> AEIGGDHGYNATNIA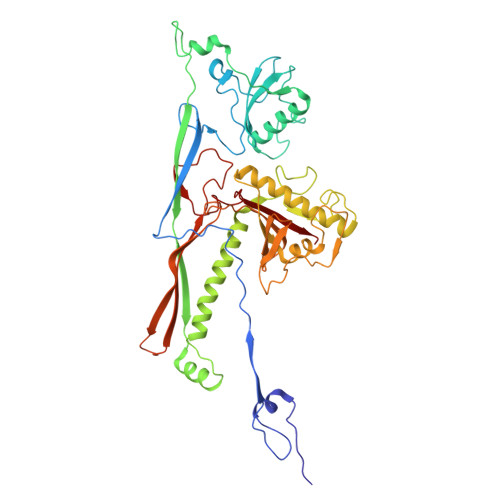AGQTSGAVTQIGPAVMGMVRRAIPNLIAFDICGVQPMNSPTGQVFALRAVYGKDPVAAGAKEAFHPMYGPDAMFSGQGAAKKFPALAASTQTTVGDIYTHFFQETGTVYLQASVQVTIDAGDEDEDEDEDATDAAKLDAEIKKQMEAGALVEIAEGMATSIAELQEGFNGSTDNPWNEMGFRIDKQVIEAKSRQLKAAYSIELAQDLRAVHGMDADAELSGILATEIMLEINREVVDWINYSAQVGKSGMTLTPGSKAGVFDFQDPIDIRGARWAGESFKALLFQIDKEAVEIARQTGRGEGNFIIASRNVVNVLASVDTGISYAAQGLATGFSTDTTKSVFAGVLGGKYRVYIDQYAKQDYFTVGYKGPNEMDAGIYYAPYVALTPLRGSDPKNFQPVMGFKTRYGIGINPFAESAAQAPASRIQSGMPSILNSLGKNAYFRRVYVKGI> MALVYDAEFVGSEREFEEERETFLKGVKAYDGVLATRYLMERSSSAKNDEELLELHQNFILLTGSYACSIDPTEDRYQNVIVRGVNFDERVQRLSTGGSPARYAIVYRRGWRAIAKALDIDEEDVPAIEVRAVKRNPLQPALYRILVRYGRVDLMPVTVDEVPPEMAGEFERLIERYDVPIDEKEERILEILRENPWTPHDEIARRLGLSVSEVEGEKDPESSGIYSLWSRVVVNIEYDERTAKRHVKRRDRLLEEL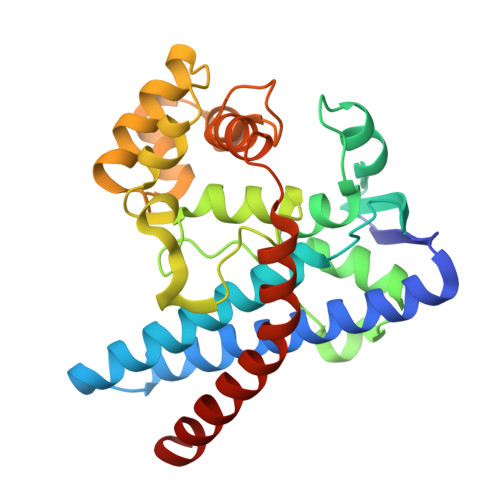YEHLEELSERYL>[2x]HDPLTGLPNRRYFFELGNRYLDLAKREGKKVFVLFVDLAGFKAINDTYGHLSGDEVLKTVSKRILDRVRRSDVVARYGGDEFTILLYDMKEEYLKSLLERILSTFREPVRVENKHLSVTPNIGVARFPEDGENLEELLKVADMRMYKAKEMKVPYFSLSLEHHHHHH

We report the structure of tDGC from Thermotoga maritima, an important enzyme for the large scale enzymatic synthesis of c-di-GMP and the first GGDEF domain from a hyperthermophile. We expressed and crystallized a domain of the TM1788 protein from Thermotoga maritima (248 residues, WP_010865403) spanning residues 82–248, hereafter named tDGC. Cellular levels of c-di-GMP are tightly regulated by the opposing activities of diguanylate cyclases (DGCs) that synthesize c-di-GMP from two GTP molecules and phosphodiesterases (PDEs) that hydrolyze c-di-GMP into 5′-phosphoguanylyl- (3′-5′) - guanosine (pGpG) and GMP. C-di-GMP synthesis from two separate GTP molecules requires dimerization of two active GGDEF domains, with the loops bearing the GGDEF motifs of each monomer brought in close proximity to initiate the cyclization reaction.

In order to understand the structural determinants of tDGC thermostability and to investigate the catalytic mechanism and feedback inhibition of this biotechnologically important enzyme, we crystallized tDGC (i) in an active-like conformation with two A-sites in proximity, and (ii) in an inactive conformation, with c-di-GMP bound to the I-site. A comparison between these two structures enables us to examine potential conformational changes propagated between the I- and A- site upon c-diGMP binding to the I-site. In conclusion, our study identified a dimeric active-like conformation for a thermostable GGDEF domain, where the relative orientation of both active sites is compatible with c-di-GMP formation. Using the tDGC active-like dimer as a guide, we were also able to propose a 2-fold symmetrical dimer conducive to GTP cyclization with a nucleophilic attack by the 3′ oxygen groups of the ribose. Further structural and enzymatic studies are now needed to confirm this model. To investigate if c-di-GMP binding at the I-site causes conformational changes at the A-site, the structures of the active-like and inactive dimer were compared. The backbone and side-chain conformations are closely similar, suggesting the absence of signal propagation between the A- and I-sites, upon c-di-GMP binding.>[3x]MDFRIGQGYDVHQLVPGRPL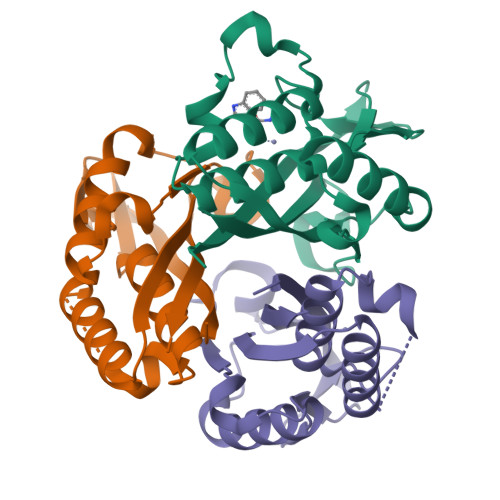IIGGVTIPYERGLLGHSDADVLLHAITDALFGAAALGDIGRHFSDTDPRFKGADSRALLRECASRVAQAGFAIRNVDSTIIAQAPKLAPHIDAMRANIAADLDLPLDRVNVKAKTNEKLGYLGRGEGIEAQAAALVVR>[2x]MSAQSALSGLGAKLLSGEVEVVDCTGVLGPNTPILQLPPDFAKNTPKVEIHKISEYDSDGPFFAWNWMVLGEHSGTHFDAPHHWITGKDYSDGFTDTLDVQRLIAPVNVIDCSKESAADPDFLLTADLIKAWEAEHGEIGAGEWVVMRTDWDKRAGDEAAFLNADETGPHSPGPTPDAIEYLLSKKIVG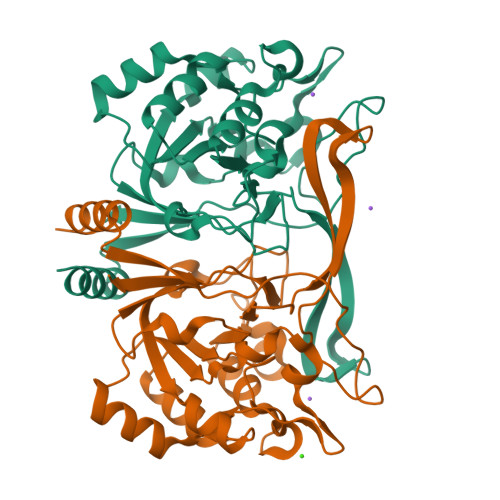WGSQCIGTDAGQAGGMEPPFPAHNLLHRDNCFGLASLANLDKLPAKGAILIAAPLKIERGTGSPIRALALVPKA> GHMSLSVAE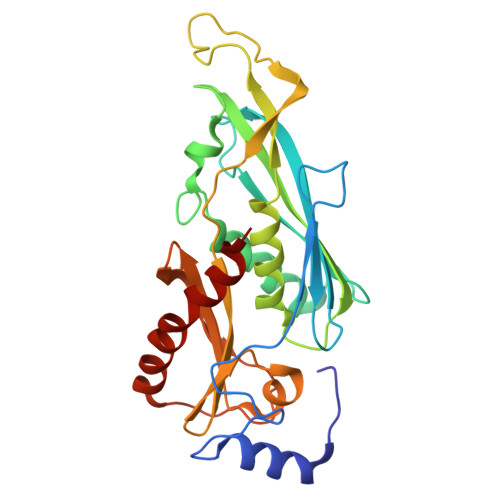KSYLYDSLASTPSIRPDGRLPHQFRPIEIFTDFLPSSNGSSRIIASDGSECIVSIKSKVVDHHVENELLQVDVDIAGQRDDALVVETITSLLNKVLKSGSGVDSSKLQLTKKYSFKIFVDVLVISSHSHPISLISFAIYSALNSTYLPKLISAFDDLEVEELPTFHDYDMVKLDINPPLVFILAVVGNNMLLDPAANESEVANNGLIISWSNGKITSPIRSVALNDSNVKSFKPHLLKQGLAMVEKYAPDVVRSLENL>[2x]MGSSHHHHHHSQDPAEKQKHDGRVKIGHYVLGDTLGVGTFGKVKIGEHQLTGHKVAVKILNRQKIRSLDVVGKIKREIQNLKLFRHPHIIKLYQVISTPTDFFMVMEYVSGGELFDYICKHGRVEEMEARRLFQQILSAVDYCHRHMVVHRDLKPENVLLDAHMNAKIADFGLSNMMSDGEFLRTSCGSPNYAAPEVISGRLYAGPEVDIWSCGVILYALLCGTLPFDDEHVPTLFKKIRGGVFYIPEYLNRSVATLLMHMLQVDPLKRATIKDIREHEWFKQGLPSYLFPEDPSYDANVIDDEAVKEVCEKFECTESEVMNSLYSGDPQDQLAVAYHLIIDNRRIMNQASEFYLASSPPSGSFMDDSAMHIPPGLKPHPERMPPLIADSPKARCPLDALNTTKPKSLAVKKAKWHLGIRSQSKPYDIMAEVYRAMKQLDFEWKVVNAYHLRVRRKNPVTGNYVKMSLQLYLVDNRSYLLDFKSIDDEVVEQRSGSSTPQRSCSAAGLHRPRSSFDSTTAESHSLSGSLTGSLTGSTLSSVSPRLGSHTMDFFEMCASLITTLAR;>[2x]MGNTSSERAALERHGGHKTPRRDSSGGTKDGDRPKILMDSPEDADLFHSEEIKAPEKEEFLAWQHDLEVNDKAPAQARPTVFRWTGGGKEVYLSGSFNNWSKLPLTRSHNNFVAILDLPEGEHQYKFFVDGQWTHDPSEPIVTSQLGTVNNIIQVKKTDFEVFDALMVDSQKCSDVSELSSSPPGPYHQEPYVCKPEERFRAPPILPPHLLQVILNKDTGISCDPALLPEPNHVMLNHLYALSIKDGVMVLSATHRYKKKYVTTLLYKPI;>[2x]MADLNWETVISSDSSPAVENEHPQETPESNNSVYTSFMKSHRCYDLIPTSSKLVVFDTSLQVKKAFFALVTNGVRAAPLWDSKKQSFVGMLTITDFINILHRYYKSALVQIYELEEHKIETWREVYLQDSFKPLVCISPNASLFDAVSSLIRNKIHRLPVIDPESGNTLYILTHKRILKFLKLFITEFPKPEFMSKSLEELQIGTYANIAMVRTTTPVYVALGIFVQHRVSALPVVDEKGRVVDIYSKFDVINLAAEKTYNNLDVSVTKALQHRSHYFEGVLKCYLHETLETIINRLVEAEVHRLVVVDENDVVKGIVSLSDILQALVLTGGEKKP

AMP-activated protein kinase (AMPK) is a conserved serine/threonine protein kinase that acts as a metabolic fuel sensor and is crucial for maintaining cellular energy homeostasis. It is a heterotrimer composed of a catalytic α subunit, an N-terminally myristoylated regulatory β subunit and a nucleotide-sensing γ subunit, each with multiple isoforms (α1, α2, β1, β2, γ1, γ2, γ3) providing the potential to form 12 distinct complexes. The capacity of AMPK to monitor cellular energy status is provided by three exchangeable adenine nucleotide binding sites on the γ-subunit. Biochemical and structural analyses reveal that many of these direct activators bind to a hydrophobic pocket located between the AMPK α kinase domain and β carbohydrate binding module (CBM), termed the Allosteric Drug and Metabolite (ADaM) site, as it can also be occupied by regulatory endogenous metabolites such as palmitoyl-CoA.

To structurally characterise the MSG011/AMPK interaction and investigate chemistry for blocking β1 binding we solved the co-crystal structure of activated α2β1γ1 (phosphorylated on α2-Thr172 and β1-Ser108) in complex with MSG011 at a resolution of 2.95 Å. As expected, MSG011 was docked in the ADaM site where clear electron density was observed for the drug in both AMPK heterotrimers in the asymmetric unit. Both MSG011 molecules were built in similar poses, however, missing electron density around the 2-methylbenzoic acid indicates flexibility in this region. Interestingly, α2-Lys29 is in close proximity to this ring and was unable to be completely modelled due to poor electron density around the ε-amino group, hence it is plausible that it is participating in both hydrophobic interactions with the 2-methylbenzoic acid of MSG011 through the hydrophobic carbon tail, and hydrogen bonding with phosphorylated β1-Ser108 through its positively charged ε-amino group. There is also flexibility around the acetamido group, which was modelled in different conformations in each heterotrimer. This chemical group is not present in previously published ADaM site-directed activators and occupies a novel space at the entrance of the ADaM site, however it does not appear to interact with any AMPK residues that are resolved in this structure. MSG011 differs from the α2 selective SC4 only in the LHS terminal ring, with addition of an acetamido and loss of aromaticity and a 2-hydroxyl group. We previously showed that the SC4 2-hydroxyl forms hydrogen bonding with α2-Lys31, suggesting that loss of this interaction confers MSG011 with the ability to activate all AMPK complexes, and conversely that the 2-hydroxyl group is important for α2 selectivity of ADaM site compounds.>[2x]SVKSEYAEAAAVGQEAVAVFNTMKAAFQNGDKEAVAQYLARLASLYTRAEELLNRILE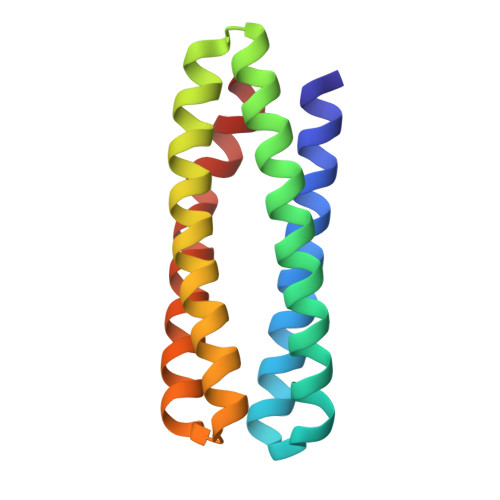KARREGNKEAVTLMNEFTATFQTGKSIFNAMVAAFKNGDDDSFESYLQALEKVTAKGETLADQIAKAL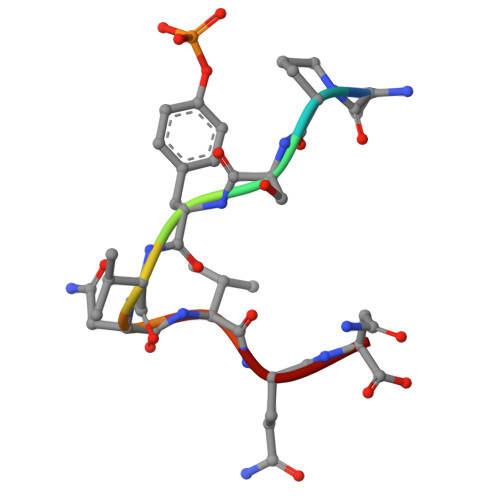> APSYVNVQN>MIRGSSALKSLTSRRLYSTGVKYTTLSNGVTVATETNPAAKTSSVGLFFGAGSRSEHSHSNGISALTTNVLASQSAKGSLLTAKNDREFNGIIAQTTNDNITEAGKLIASIASNAVDIVEKTDLTKHKQYLSAQASAVEADPKSKVLSHLYSSAFQGYSLALPTLGTTESVENLENQDSLRHLAKHLVNNNTVIAASGNFDHDKLADAIEANLKIAEGVKPEIKPASFLGSEVRMRDDTLPKAYISIAVHGEGLNSPNYYLAKVAAAIYGDFYLHSTIAKFTSPKLASIVQEYNIVESYNHYSKSFSDTGIWGYYAEIADKFTVDDFTHFSLKEWNRLSISISEAEVARAKAQVKTALAKELANSFAVTSDIAEKVLLVGHRQSLREAFEKIDAIKVNDVKEWGKSKVWDRDIVISGTGLIEDLLDYNRNRNEMAMMRW[2x];>[2x]MLSRASIRAYSSIPNSVKIAAKESATDLTKLSVIINNAGSKTGKSGVSHLLSKFTFLNNGAKSALRFTRESELLGGTFESKVTRDALILNTTFLKQDLPYYVEALGNVVSNTQFAPHEFNEIVLPTANAETKLANANPAFKGVEKLHEITFRRGLGNPLFYNESTPIKLEEVAQFSKEQFSGENISIVAEGANEEDLTKFVSESAFCYLPSSSSNGAKALPTNTFTGQEARVPSSGASSALIGIPVKPADFGKYEVLSAAIGTSTLPSTSTPLAQIPGATSHLYKYQDAGLFVISVSGEASQVAQGIKQAKSVAESVSSSALSEAVKAAELSVALQSTVDSPLNVKVVAEEAPISKFNYVAVGDLDVLPYADEL;>MSSLAFRTLRNGLGLKSSVRALSTTTTTLSNYQQPDYSSYLNNKSGQGSRNFTYFMVGSMGLLSAAGAKSTVEAFLSSFAASADVLAMAKVEVKLGAIPEGKNVIIKWQGKPVFIRHRTADEIEEANQVDIKTLRDPQNDADRVKKPEWLIMLGICTHLGCVPIGEAGDFGGWFCPCHGSHYDISGRIRKGPAPLNLEIPEYDFTDDETLLVG[2x];>MFRTAYKTMNQSMVQKFIAGGVGVTGLTASYLLYQDSMTADAMTAAEHGLHPPAYNWPHNGMFETFDHASIRRGFQVYREVCAACHSLDRIAWRNLVGVSHTTSEAKAMAEELEYDDEPDDEGKPRKRPGKLADYIPGPYENEQAARAANQGAYPPDLSLIVKARHGGSDYIFSLLTGYPDEPPAGVVLPEGSNYNPYFPGGAIAMGRVLFDDLVEYEDGTPATTSQMAKDVSTFLNWASEPEHDDRKKWGLKALVVLSSLYLLSIWVKRFKWTPIKNRKFRFDPPKK[2x];>[2x]MAGAPHPHTYMGWWGSLGSPKQKYITQYTISPYAAKPLKGAAYNAVFNTFRRTKNQFLYVAIPFVVVWSIWTRARDYNEYLYTKEGREELERVNV;>MVQSMTSVVKAANFILARPTLSKIITPLAQKFTAYAGYREMGLKFNDLLLEETPIMQTAIKRLPSELNYSRNFRILTAHQLALSHQLLPAEKAVKPEEDDNYLIPYILEAEKEAFEKAELDNIEVKA[2x];>[2x]MSFFRDLLESVVPTAYAEEPVEDVEVEQPEDAPEEEVSEETVEEEEEDDEDDDEDDEEEEETADPLDTLREECTKTAACKPFDHHFHECIERVTKEQEEPDYEHKHYKEDCIEEFFHLQHCVNDCVAPRLFNRLK;>[2x]MLTVLGRLLERNSIYVATIFGGAFAFQGFFDVAVNKWWEEHNKAKLWKNVKGKFLEGEGEEEDDE;>MPTRKSNTYLSLVNSYLIDSPQPSSINYWWNLGSLLGLCLVIQIASGVFLAMHYSSNIELAFDSVEHIMRDVNAGWLIRYIHANGASFFFICMY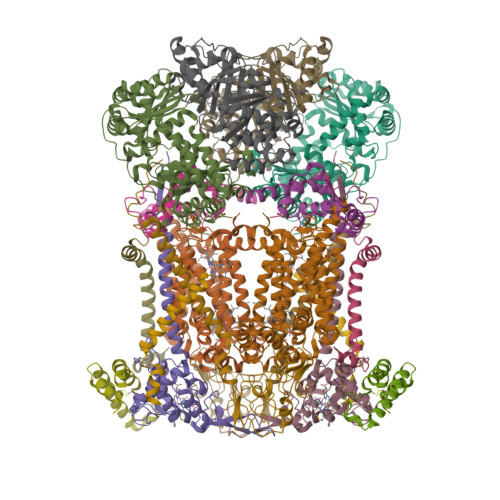LHIGKALYYGSYKQPRVMLWVIGVVIFILTMAIAFMGYCLVYGQMSHWGATVITNLLSAIPFIGNDIVPFIWGGFSVSNPTIQRFFALHFLLPFILAALVCMHLMALHVHGSSNPVGITGNIDRLPMHPYFIFKDLITVFVFLLIFSLFVFYSPNTLGHPDNYIPGNPMVTPPSIVPEWYLLPFYAILRSIPDKLGGVIAMFGAILILLSLPYTDRSIIRGNSFKVLSKLAFYLFVFNFILLGNLGQLHVEVPYIQLGQFATAYYFAHYIIVVPVISTLENILYYIGTQTRVK[2x]>SVNAATVDLRIMETTDLHSNMMDFDYYKDAATEKFGLVRTASLIEQARAEVKNSVLVDNGDVIQGSPLGDYMAAKGLKE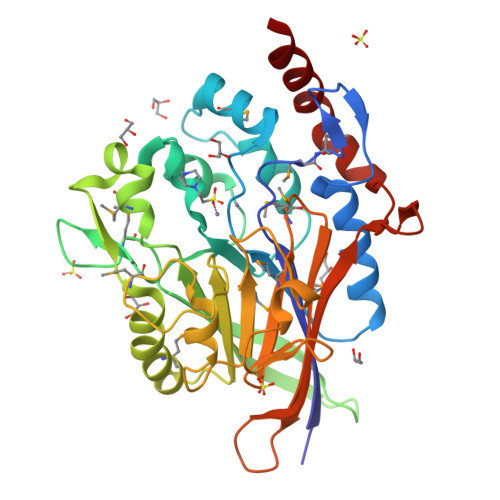GDVHPVYKAMNTLNYAVGNLGNHEFNYGLDFLHKALAGAKFPYVNANIIDAKTGKPMFTPYLIQDTRVVDSDGQIHTLRIGYIGFVPPQIMTWDKANLNGKVTVNDITETARKYIPEMRAKGADVVVVVAHSGLSADPYQAMAENSVYYLSQVPGVDAIMFGHAHAVFPGKDFANIKGADIAKGTLNGVPAVMPGMWGDHLGVVDLVLNNDSGKWQVTQSKAEARPIYDAVAKKSLAAEDGKLVSVLKADHDATREFVSK[2x]IDE can effectively degrade insulin, amylin, and glucagon, pancreatic hormones that control blood glucose levels, as well as amyloid β (Aβ), a peptide implicated in Alzheimer’s disease. IDE is a 110 kDa zinc metalloprotease that readily dimerizes in solution (Kd =~ 10 nM). IDE has at least two major conformational states in its catalytic cycle; open-state IDE captures substrates and releases products while closed-state IDE performs catalysis. Within the IDE dimer, each IDE subunit consists of ~55 kDa N- and C-terminal domains, IDE-N and IDE-C.

Further 3D classification revealed three major conformations and structural models were built. We again applied IDE dimer-focused classification with signal subtraction of the IDE-FabH11-E dimer to refine each conformation separately, which improved the resolution significantly. The three apo-IDE structures derive from combinations of the IDE partial open (pO) and open (O) states. The three conformers have resolution limits which correlated well with their relative populations: O/pO (4.2 Å, 73%), O/O (6.5 Å, 16%), and pO/pO (6.9 Å, 11%). Furthermore, two subunits within O/O or pO/pO states have noticeable differences in the distance and buried surface between IDE-N and IDE-C and the dihedral angle. The IDE pO and O states differs from the pC and C states by 5 Å to 24 Å increases in the distance between D1 and D4 and 7° to 17° increases in the dihedral angle, respectively. These changes result in decreased buried surface between IDE-N and IDE-C in pO and O states. By rigid-body motion between IDE-N and IDE-C, IDE switches between O and pO states. Our cryoEM data reveal that two IDE-N domains within the IDE dimer undergoes rigid body motion, allowing IDE to undergo the transition between the open and ‘closed’ states without the assistance of substrate.

>[2x]AIKRIGNHITKSPEDKREYRGLELANGIKVLLISDPTTDKSSAALDVHIGSLSDPPNIAGLSHFLEHMLFLGTKKYPKENEYSQFLSEHAGSSNAFTSGEHTNYYFDVSHEHLEGALDRFAQFFLSPLFDESAKDREVNAVDSEHEKNVMNDAWRLFQLEKATGNPKHPFSKFGTGNKYTLETRPNQEGIDVRQELLKFHSAYYSSNLMAVVVLGRESLDDLTNLVVKLFSEVENKNVPLPEFPEHPFQEEHLKQLYKIVPIKDIRNLYVTFPIPDLQKYYKSNPGHYLGHLIGHEGPGSLLSELKSKGWVNTLVGGQKEGARGFMFFIINVDLTEEGLLHVEDIILHMFQYIQKLRAEGPQEWVFQELKDLNAVAFRFKDKERPRGYTSKIAGILHYYPLEEVLTAEYLLEEFRPDLIEMVLDKLRPENVRVAIVSKSFEGKTDRTEEWYGTQYKQEAIPDEVIKKWQNADLNGKFKLPTKNEFIPTNFEILPLEKEATPYPALIKDTAMSKLWFKQDDKFFLPKANLNFEFFSPFAYVDPLHSNMAYLYLELLKDSLNEYAYAAELAGLSYDLQNTIYGMYLSVKGYNDKQPILLKKIIEKMATFEIDEKRFEIIKEAYMRSLNNFRAEQPHQHAMYYLRLLMTEVAWTKDELKEALDDVTLPRLKAFIPQLLSRLHIEALLHGNITKQAALGIMQMVEDTLIEHAHTKPLLPSQLVRYREVQLPDRGWFVYQQRNEVHNNSGIEIYYQTDMQSTSENMFLELFAQIISEPAFNTLRTKEQLGYIVFSGPRRANGIQGLRFIIQSEKPPHYLESRVEAFLITMEKSIEDMTEEAFQKHIQALAIRRLDKPKKLSAESAKYWGEIISQQYNFDRDNTEVAYLKTLTKEDIIKFYKEMLAVDAPRRHKVSVHVLAREMDSCPVVGEFPCQNDINLSQAPALPQPEVIQNMTEFKRGLPLFPLVKPH>GLPVPSPPGTLLPGQSPDEAFARNSVVFLVPGAEYNWKNVVIRKPVWIYGNGATVKTSGLGPIIHIMGDLDNPMDVRIQDLTFIGGDSPDRLVPFSAVLTNQMALWCIDPRITIRGCSFYNFGGAAIYLERSERDTGFRFGRGQVMITDCRFRGCRIGIANGGSVEYGLASQNNFSDCQICFNVVGGNWTRSGNVASNCRCMYLHTQGMWYEGAAGNFNPAHGSFTSNTLNHCDYGGNLW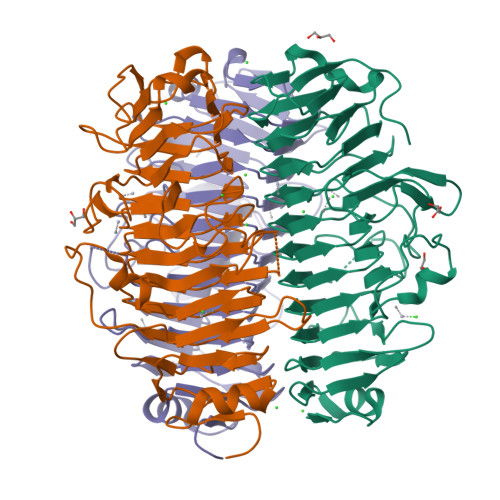PTEFQLPDRVINLAGFYFDNAAARLPNFSGNSQWYGDMKLINFLPDSTFVINGGALYGGPGDTGVIAVATALAAKVFVIGCQGNAGQQIVNVPAANIIPEVGTRKDDATQPAA[3x]> EGTAFARSEGASALASVNPLKTTVEE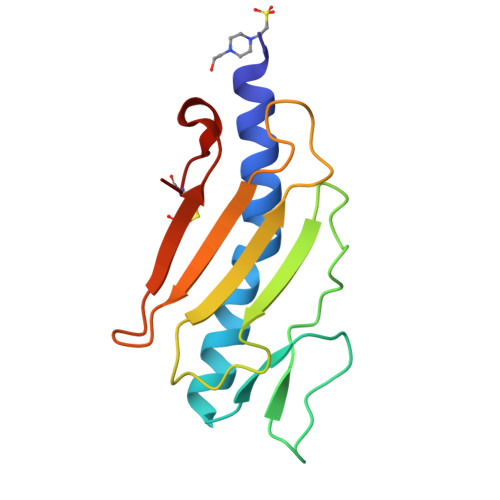ALSRGWSVKSGTGTEDATKKEVPLGVAADANKLGTIALKPDPADGTADITLTFTMGGAGPKNKGKIITLTRTAADGLWKCKSDQDPQFIPKGCS>GMVRIAVAGAAGRMGRNLVKAAHHNPVAKVAAGSERPESSLVGVDLGELCGEGKFDVVVCDDLAKQIDQFDVIIDFTAPASTLNNLALCQQYGKSIVIGTTGFTEEQREQIDLVAQQVPVVMAPNYSVGVNLVFKLLEKAAKVMGDYCDIEIVEAHHRHKVDAPSGTAIGMGEAIAGAMGNKLSDVAVYAREGITGERTKDEIGFATIRAGDIVGEHTAMFADIGER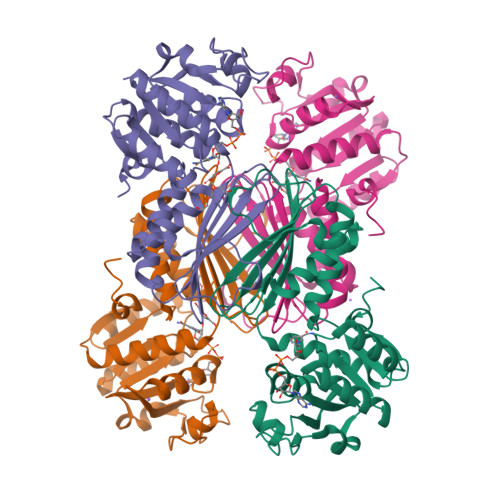VEITHKATDRMTFANGAVKAAVWLHEKPAGFYTMTDVLGLNDL[4x]> MSREQIIKDGGNILVTAGAGSGKTTILVSKIEADLKENKTHYSIAAVTFTNKAAKEIEGRLGYSSRGNFIGTNDGFVESEIIRPFIKDAFGNDYPDNFTAEYFDNQFASYDKGLQVLKYQNILGTYSNPKKNFKFQLALDILKKSLVARQYIFSKYFKIFIDEYQDSDKDMHNLFMYLKDQLKIKLFIVGDPKQSIYIWRGAEPENFNGLIENSTDFNKYHLTSNFRCCQDIQNYSNLFNEETRSLIKEKNEVQNVISIADDMPISDILLKLTEEKQVLNIEAELVILVRRRNQAIEIMKELNEEGFNFIFIPQTPLDRATPNATLLKEVIKYVKNDRYSIYDLAAEIVGNLSSREIKEIQKIINELLVPNINQVLINQVLINLFAKLEITLDTREITAFT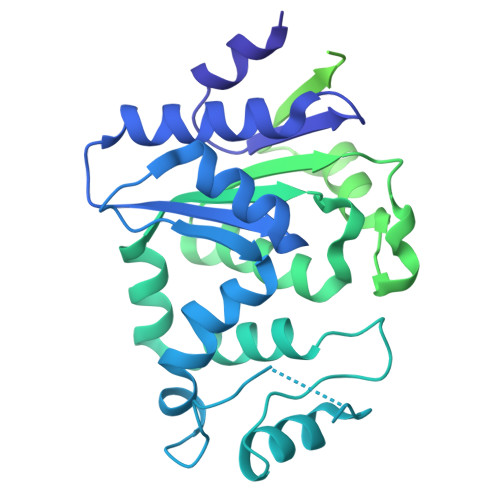EVMMTNEFDIAFDTNEYLHKIFTVHSAKGLEFNQVIITASDYNVHYNRDTNEHYVATTRAKDKLIVIMDNKKYSDYIETLMKELKIKNIIKSI5-azanyl-1,2-dihydropyrazol-3-one 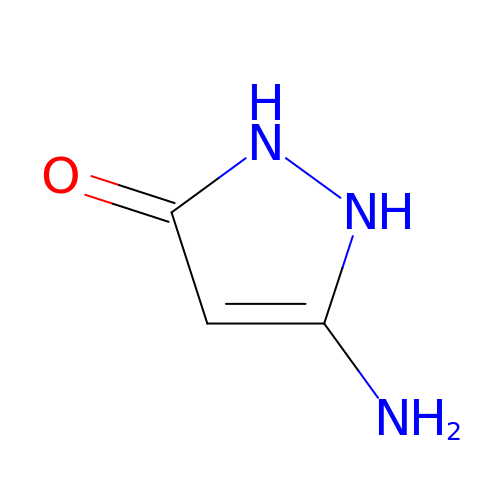| C3 H5 N3 O | QZBGOTVBHYKUDS-UHFFFAOYSA-N>GSHMDNQCT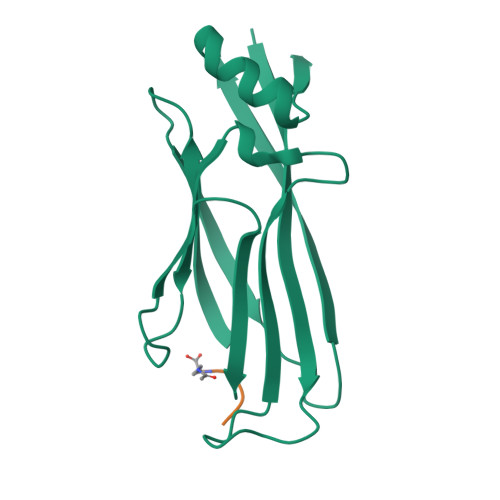VQVRLELGHRAQLRKKPTTEGFTHDWMVFVRGPEQCDIQHFVEKVVFWLHDSFPKPRRVCKEPPYKVEESGYAGFIMPIEVHFKNKEEPRKVCFTYDLFLNLEGKVNHLRCEKLTFNNPTTEFRYKLLRAGGVMVMPEGAHHHHHH[4x];>[4x]AARK>[6x]HSWERLAVLVLLGAAACAAPPRGRILGGREAEAHARPYMASVQLNGAHLCGGVLVAEQWVLSAAHCLEDAADGKVQVLLGAHSLSQPEPSKRLYDVLRAVPHPDSQPDTIDHDLLLLQLSEKATLGPAVRPLPWQRVDRDVAPGTLCDVAGWGIVNHAGRRPDSLQHVLLPVLDRATCNRRTHHDGAITERLMCAESNRRDS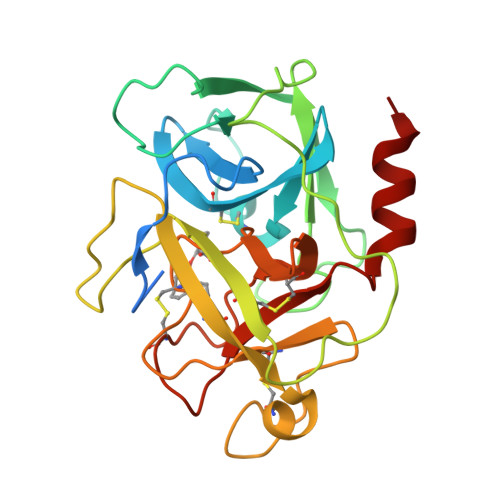CKGDSGGPLVCGGVLEGVVTSGSRVCGNRKKPGIYTRVASYAAWIDSVLASA N-(2,2-difluoro-5H-[1,3]dioxolo[4,5-f]benzimidazol-6-yl)-2-{[2-(trifluoromethoxy)benzoyl]amino}-1,3-thiazole-4-carboxamide | 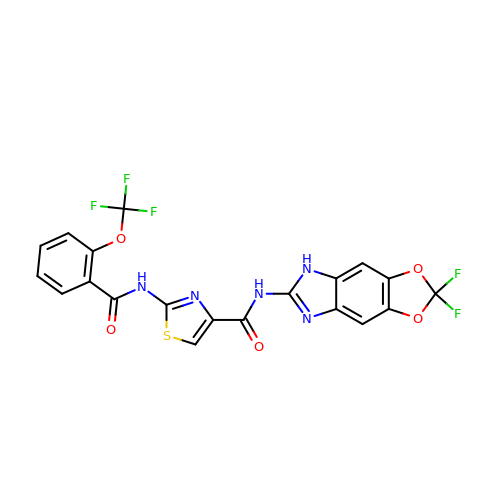C20 H10 F5 N5 O5 S | DVVVOLSRHWJCHV-UHFFFAOYSA-N> GAMDPKVTMNDFDYLKLLGKGTFGKVILVREKATGRYYAM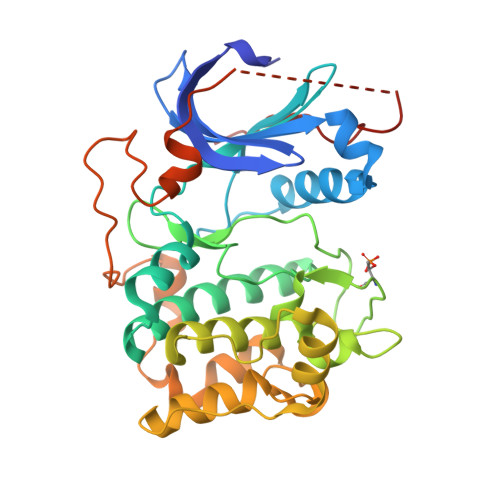KILRKEVIIAKDEVAHTVTESRVLQNTRHPFLTALKYAFQTHDRLCFVMEYANGGELFFHLSRERVFTEERARFYGAEIVSALEYLHSRDVVYRDIKLENLMLDKDGHIKITDFGLCKEGISDGATMKTFCGTPEYLAPEVLEDNDYGRAVDWWGLGVVMYEMMCGRLPFYNQDHERLFELILMEEIRFPRTLSPEAKSLLAGLLKKDPKQRLGGGPSDAKEVMEHRFFLSINWQDVVQKKLLPPFKPQVTSEVDTRYFDDEFTAQSITITPPDRYDSLGLLELDQREEQEMFEDFDYIADW>[4x]ASMTGGQQMGRDEAGI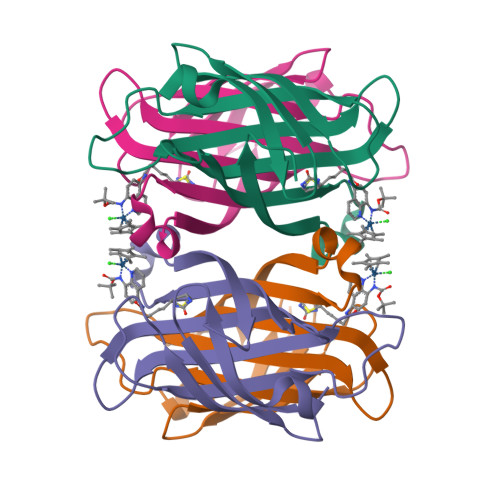TGTWYNQLGSTFIVTAGADGALTGTYESAVGNAESRYVLTGRYDSAPATDGSGTALGWTVAWKNNYRNAHSATTWSGQYVGGAEARINTQWLLTIGTTEANAWKSTLVGHDTFTKVKPSAASIDAAKKAGVNNGNPLDAVQQ>[3x]ETGEATKSVSKTEHAEINIFSVASGHLYERMLNIMMASVMHHTNHTVKFWFIEQFLSPSFKDFIPHMAAEYGFKYEMVTYKWPHWLRQQKEKQREIWGYKILFLDVLFPLSLDKVIFVDADQIVRTDMYDL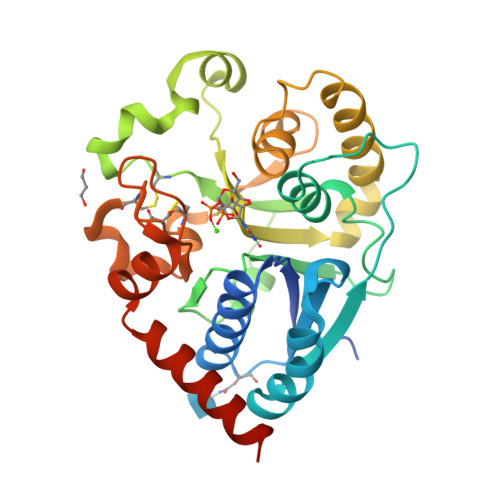VEHPLDGAPYGFAPMCDSRVEMEGYRFWKTGYWANYLKGKPYHISALYVVDLQRFRELAAGDRLRQQYHALSADPNSLANLDQDLPNHMQFTIPIATLPQEWLWCETWCSDETLKDARTIDLCNNPMTKEPKLDRARRQVPEWTKYDEEIAELARRVREGTKHHHH> GMYQTIEGFLQSWTYETESTQKMLDVLTDESLSQEIAPGHWTLGRVAWHIVTAIPVILSGTGLKFEGETKDYPVPTSAKTIADGYRKVNTAFVEALQSEWTDKDLTTINDFFGRPMPNS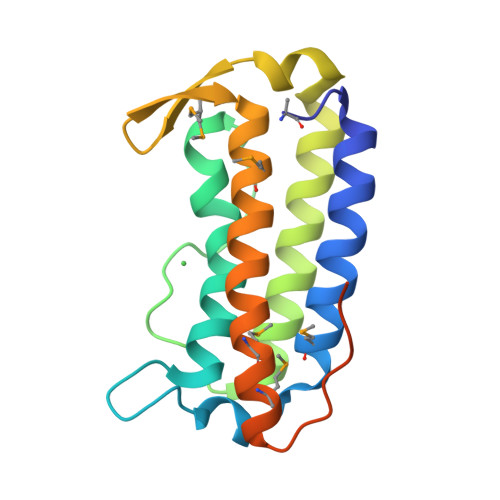IFLMTLINHQNHHRGQMTVLMRQAGLTVPGVYGPAKEEWATAGMEAPKM>MHHHHHHNSITSATDEQPHIGNYRLQKTIGKGNFAKVKLARHVLTGREVAVKIIDKTQLNPTSLQKLFREVRIMKILNHPNIVKLFEVIETEKTLYLVMEYASGGEVFDYLVAHGRMKEKEARAKFRQIVSAVQYCHQKYIVHRDLKAENLLLDGDMNIKIADFGFSNEFTVGNKLDEFCGSPPYAAPELFQGKKYDGPEVDVWSLGVILYTLVSGSLPFDGQNLKELRERVLRGKYRIPFYMSTDCENLLKKLLVLNPIKRGSLEQIMKDRWMNVGHEEEELKPYTEPDPDFNDTKRIDIMVTMGFARDEINDALINQKYDEVMATYILLGRKPPEFEGGESLSGEPKERDKEEGKDSKPRSLRFTWSMKTTSSMDPNDMMREIRKVLDANNCDYEQKERFLLFCVHG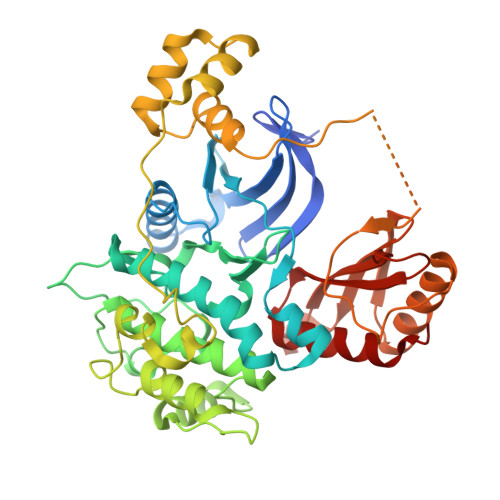DARQDSLVQWEMEVCSLPSLSLNGVRFKRISGTSIAFKNIASKIANELKL[2x]> GHMASNEDFKDWADPQSNPQEESAGQLTATFTAGKDASIVMDAATADSVEIAKLSSTTAEEGSKIAVNSLTLNENHTIPFSMTEDHVFKVALAQLDSVTQ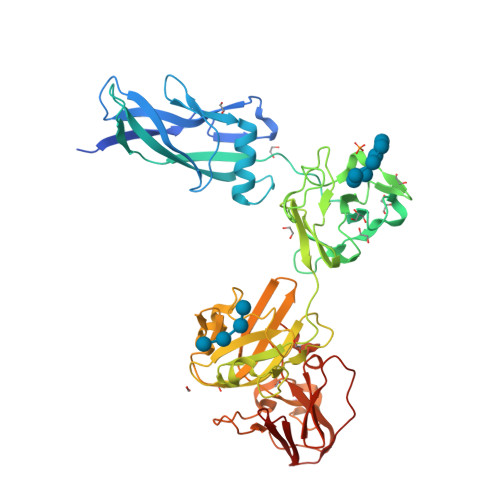EAYKSRASVVRELKISINASAVTPSGEGIQLVGNEVSITLQPATTPAVDPDGYYIVGDFTGWDGNSAQQMKKDALDENLYILEAEIESTSNFKIFPASAINGNDIDWTKALGSSVDGDDSGDNFVSWTNAGAINTALDGKIKISFDAFNYRFTVKDNSAPTELYMTGSAYNWGTPAGDPNAWKALVPVNGTKGTFWGIFYFAANDQVKFAPQANWGNDFGFVDAISQESKDLAGLSDEGGNLKVGIAGWYLVYVSVIGDDKVIEFEKPNVYLMGDTSYNGWDAQLVEQDLFTVPGTADGEFVSPAFLKDGAVRICVNPKAVSAGDWWKTEFIIFDGQIAYRGNGGDQAAVQGKTGQKVYLNFGNGTGRIE>MAKIYKDEDISLEPIKNKTIAILGYGSQGRAWALNLRDSGLNVVVGLERQGDSWRRAIDDGFKPMYTKDAVAIADIIVFLVPDMVQKSLWLNSVKDFMKKGADLVFAHGFNIHFKIIEPPKDSDVYMIAPKSPGPIVRRSYEMGGGVPALVAVYQNVSGEALQKALAIAKGIGCARAGVIESTFKEETETDLFGEQVILVGGIMELIKASFETLVEEGYQPEVAYFETVNELKLIVDLIYEKGLTGMLRAVSDTAKYGGITVGKFIIDKSVRDKMKIVLERIRSGEFAREWIKEYERGMPTVFKELSELEGSTIETVGRKLREMMFRGMKQISSH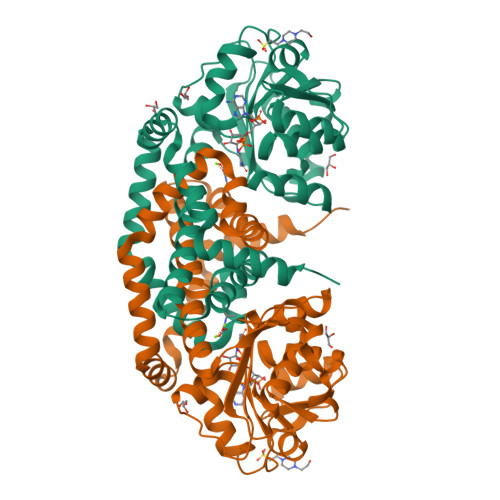LEHHHHHH[2x]> PFEIVFEGAKEFA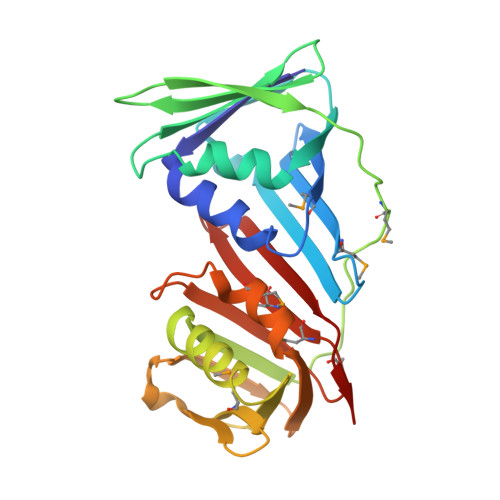QLIDTASKLIDEAAFKVTEDGISMRAMDPSRVVLIDLNLPSSIFSKYEVVEPETIGVNLDHLKKILKRGKAKDTLILKKGEENFLEITIQGTATRTFRVPLIDVEEMEVDLPELPFTAKVVVLGEVLKAAVKAASLVSDSIKFIARENEFIMKAEGETQEVEIKLTLEDEGLLDIEVQEETKSAYGVSYLSDMVKGLGKADEVTIKFGNEMPMQMEYYIRDEGRLTFLLAPRVEE> FACKTANGT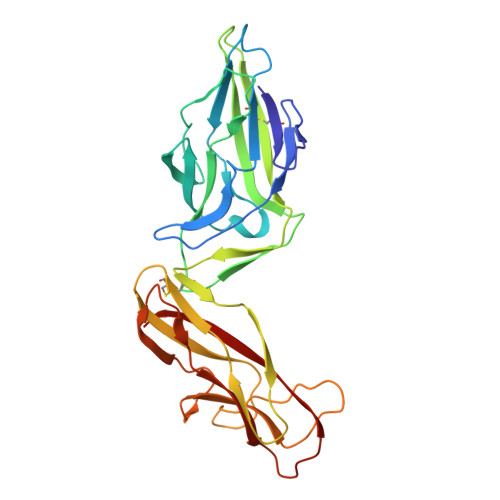AIPIGGGSANVYVNLAPAVNVGQNLVVDLSTQIFCHNDYPETITDYVTLQRGSAYGGVLSSFSGTVKYNGSSYPFPTTSETPRVVYNSRTDKPWPVALYLTPVSSAGGVAIKAGSLIAVLILRQTNNYNSDDFQFVWNIYANNDVVVPTGGCDVSARDVTVTLPDYPGSVPIPLTVRCDQTQSVSYTLSGSVADAGNSIFTNTASFSPAQGVGVQLTRNGTIIPANNTVSLGAVGTSAVSLGLTANYARTGGQVTAGNVQSIIGVTFVYQ> GVGVSTGSYDNQTHYRFLGDGWVEITALATRLVHLNMPKSENYCRIRVHNTTDTSVKGNMAKDDAHEQIWTPWSLVDANAWGVWLQPSDWQYICNTMSQLNLVSLDQEIFNVVLKTVTEQDLGGQAIKIYNNDLTACMMVAVDSNNILPYTPAANSMETLGFYPWKPTIASPYRYYFCVDRDLSVTYENQEGTVEHNVMGTPKGMNSQFFTIENTQQITLLRTGDEFATGTYYFDTNPVKLTHTWQTNRQLGQPPLLSTFPEADTDAGTLTAQGSRHGTTQMGVNWVSEAIRTRPAQVGFCQPHNDFEASRAGPFAAPKV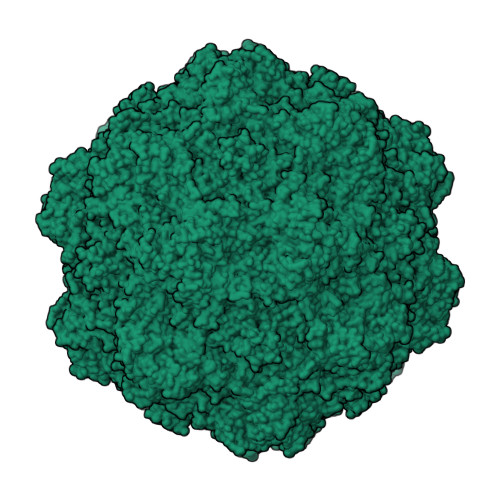PADITQGVDKEANGSVRYSYGKQHGENWASHGPAPERYTWDETSFGSGRDTKDGFIQSAPLVVPPPLNGILTNANPIGTKNDIHFSNVFNSYGPLTAFSHPSPVYPQGQIWDKELDLEHKPRLHITAPFVCKNNAPGQMLVRLGPNLTDQYDPNGATLSRIVTYGTFFWKGKLTMRAKLRANTTWNPVYQVSAEDNGNSYMSVTKWLPTATGNMQSVPLITRPVARNTY methyl (1S,3S)-1-methyl-3-[[3-[[3-methyl-4-[(4-pyridin-3-ylpyrimidin-2-yl)amino]phenyl]carbamoyl]phenyl]carbamoyl]-4-oxidanylidene-cyclohexane-1-carboxylate 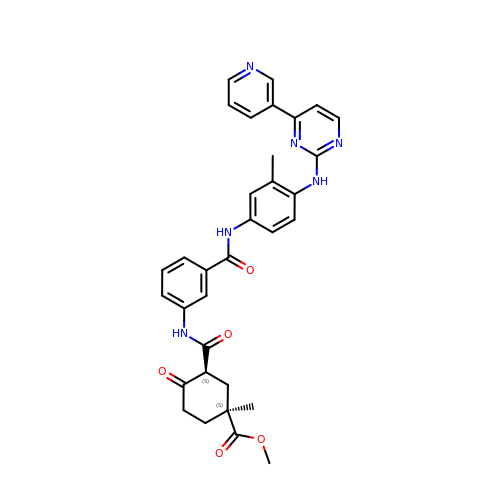| C33 H32 N6 O5 | LOKFZRXMKAWKTK-JQJBXXCASA-N> MDRASELLFYVNGRKVIEKNVDPETMLLPYLRKKLRLTGTKYGCGGGGCGACTVMISRYNPITKRIRHHPANACLIPICSLYGAAVTTVEGIGSTHTRIHPVQERIAKCHGTQCGFCTPGMVMSIYTLLRNHPEPTLDQLTDALGGNLCRCTGYRPIIDACKTFCKTSGCCQSKENGVCCLDQGINGLPEFEEGSKTSPKLFAEEEFLPLDPTQELIFPPELMIMAEKQSQRTRVFGSERMMWFSPVTLKELLEFKFKYPQAPVIMGNTSVGPEVKFKGVFHPVIISPDRIEELSVVNHAYNGLTLGAGLSLAQVKDILADVVQKLPEEKTQMYHALLKHLGTLAGSQIRNMASLGGHIISRHPDSDLNPILAVGNCTLNLLSKEG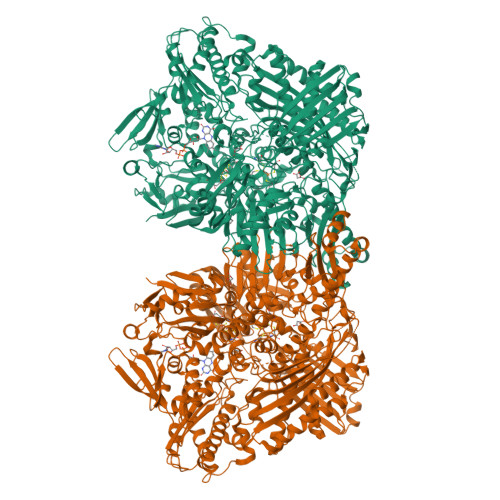KRQIPLNEQFLSKCPNADLKPQEILVSVNIPYSRKWEFVSAFRQAQRQENALAIVNSGMRVFFGEGDGIIRELCISYGGVGPATICAKNSCQKLIGRHWNEQMLDIACRLILNEVSLLGSAPGGKVEFKRTLIISFLFKFYLEVSQILKKMDPVHYPSLADKYESALEDLHSKHHCSTLKYQNIGPKQHPEDPIGHPIMHLSGVKHATGEAIYCDDMPLVDQELFLTFVTSSRAHAKIVSIDLSEALSMPGVVDIMTAEHLSDVNSFCFFTEAEKFLATDKVFCVGQLVCAVLADSEVQAKRAAKRVKIVYQDLEPLILTIEESIQHNSSFKPERKLEYGNVDEAFKVVDQILEGEIHMGGQEHFYMETQSMLVVPKGEDQEMDVYVSTQFPKYIQDIVASTLKLPANKVMCHVRRVGGAFGGKVLKTGIIAAVTAFAANKHGRAVRCVLERGEDMLITGGRHPYLGKYKAGFMNDGRILALDMEHYSNAGASLDESLFVIEMGLLKMDNAYKFPNLRCRGWACRTNLPSNTAFRGFGFPQAALITESCITEVAAKCGLSPEKVRIINMYKEIDQTPYKQEINAKNLIQCWRECMAMSSYSLRKVAVEKFNAENYWKKKGLAMVPLKFPVGLGSRAAGQAAALVHIYLDGSVLVTHGGIEMGQGVHTKMIQVVSRELRMPMSNVHLRGTSTETVPNANISGGSVVADLNGLAVKDACQTLLKRLEPIISKNPKGTWKDWAQTAFDESINLSAVGYFRGYESDMNWEKGEGQPFEYFVYGAACSEVEIDCLTGDHKNIRTDIVMDVGCSINPAIDIGQIEGAFIQGMGLYTIEELNYSPQGILHTRGPDQYKIPAICDMPTELHIALLPPSQNSNTLYSSKGLRESGVFLGCSVFFAIHDAVSAARQERGLHGPLTLNSPLTPEKIRMACEDKFTKMIPRDEPGSYVPWNVPI> MEGEGRGRWALGLLRTFDAGEFAGWEKVGSGGFGQVYKVRHVHWKTWLAIKCSPSLHVDDRERMELLEEAKKMEMAKFRYILPVYGICQEPVGLVMEYMETGSLEKLLASEPLPWDLRFRIVHETAVGMNFLHCMSPPLLHLNLKPANILLDAHYHVKISDFGLAKCNGMSHSHDLSMDGLFGTIAYLPPERIREKSRLFDTKHDVYSFAIVIWGVLTQKKPFADEKNILHIMMKVVKGHRPELPPICRPRPRACASLIGLMQRCWHADPQVRPTFQEITSETEDLCEKPDEEVKDLAHEPGEKSSLESKSEARPESSRLKRASAPPFDNDCSLSELLS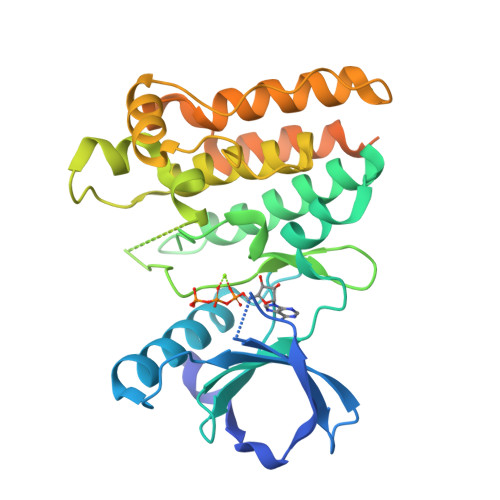QLD PALS1 regulates cell polarity through binding to the PDZ-binding domain (PBM) of CRB3 with loss of PALS1 leading to disruption of cell polarity including loss of integrity of tight and adherens junctions. Importantly, the SARS-CoV-1 E protein’s PDZ-binding motif13 sequence allows interaction with the host cell polarity signalling protein PALS1 (Protein associated with Lin7/MPP5) thus interfering with epithelial function and integrity, a property of the SARS-CoV-1 E protein which is thought to be important for its virulence. As previously shown the PALS1 PDZ domains adopts a compact globular fold comprising five to six β‐strands and two α‐helices that form a β‐sandwich structure. Examination of both the PALS1 PDZ:SARS-CoV-1_E and PALS1 PDZ:SARS-CoV-2_E complexes showed that the E protein PBM peptides are bound in the canonical ligand-binding groove formed by the β2 strand and helix α2.

To understand the structural basis of the PALS1 PDZ and SARS-CoV-1/2 E PBM interaction, we determined the crystal structures of PALS1 PDZ bound to the SARS-CoV-1_E (SRVPDLLV) and SARS-CoV-2_E (EGVPDLLV) PBM peptides to resolutions of 1.74 and 1.9 Å, respectively. PALS1 PDZ:SARS-CoV-1_E and PALS1 PDZ:SARS-CoV-2_E superimposed with one another yielded an overall root‐mean‐square deviation (RMSD) of 0.72 Å. Key hydrogen bond and ionic interactions between the PALS1 PDZ:SARS-CoV-2_E are identical with SARS-CoV-1_E. Major differences are found among the hydrophobic contacts, with the rotamer of SARS-CoV-1_E Leu73 differing from SARS-CoV-2_E Leu74. Furthermore, in SARS-CoV-1_E only Val75, Leu74 and Leu 73 are involved in hydrophobic contacts, whereas in SARS-CoV-2_E Pro72, Val71 are also involved in hydrophobic contacts. A comparison of our structures with apo-PALS1 PDZ reveals that similarly, both SARS-CoV-1_E and SARS-CoV-2_E binding to PALS1 PDZ trigger rotation of PALS1 Phe318 out of the ligand-binding groove to allow binding of SARS-CoV-1/2_E PBM. Our ITC measurements revealed that whilst PALS1 PDZ did not bind to MERS-CoV_E, it bound to SARS-CoV-1_E with an affinity of 29.6 μM, and SARS-CoV-2_E with an affinity of 22.8 μM. However, despite the sequence differences between SARS-CoV-1_E and SARS-CoV-2_E PBM in positions −5 and −6, affinities for PALS1 PDZ are comparable, indicating that positions 0, −1, −2 and −3 are required for CoV_E PBM interaction with PALS1 PDZ and define binding, whereas positions −4, −5, −6 and −8 do not play a major role.

>[4x]GPLGSKIVRIEKARDIPLGATVRNEMDSVIISRIVKGGAAEKSGLLHEGDEVLEINGIEIRGKDVNEVFDLLSDMHGTLTFVLIPSQ;>[4x]SRVPDLLV>GPLGSPNSEEEASVSVWDEEEDGATFTVTSRQYRPLDPLAPLPPPRSSRRLRAGTLEALVRHLLDART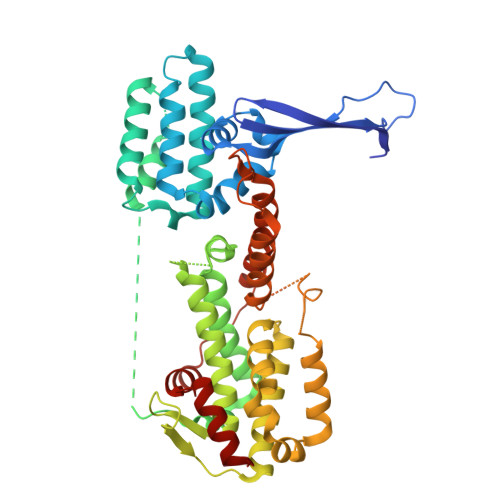AGADMMFTPALLATHRAFTSTPALFGLVADRLEALESYPPGELERTTGVAISVLSTWLASHPEDFGSEVKGQLDRLESFLLRTGYAAREGVVGGSADLIRNLRARVDPRAPDLPKPLALPGDSPADPTDVLVFLADHLAEQLTLLDAELFLNLIPSQCLGGLWGHRDRPGHSHLCPSVRATVTQFNKVAGAVVSSVLGATSIGEGPREVTVRPLRPPQRARLLEKWIRVAEECRLLRNFSSVYAVVSALQSSPIHRLRAAWGETTRDSLRVFSSLCQIFSEEDNYSQSRELLTQEVKPQPPVEPHSKKAPRSGFRGGGVVPYLGTFLKDLVMLDAASKDELENGYINFDKRRKEFAILSELLRLQKECRGYDLRPNSDIQQWLQGLQPLTEAQSHRVSCEVEPPG[2x]>MQNKIVKIGNIDVANDKPFVLFGGMNVLESRDMAMQVCEAYVKVTEKLGVPYVFKASFDKANRSSIHSYRGPGMEEGLKIFQELKDTFGVKIITDVHEIYQCQPVADVVDIIQLPAFLARQTDLVEAMAKTGAVIN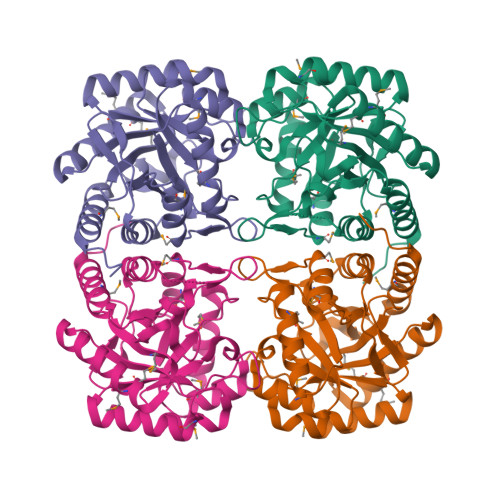VKKPQFLSPSQMGNIVEKIEECGNDKIILCDRGTNFGYDNLIVDMLGFSVMKKASKGSPVIFDVTHSLQCRDPFGAASSGRRAQVTELARSGLAVGIAGLFLEAHPNPNQAKCDGPSALPLSALEGFVSQMKAIDDLVKSFPELDTSIGSHHHHHH[4x]>[4x]GSTLKEQIGMRALNVAETVASTSLVREAFRDSNPSVRLQPFAERIRQKTGAEYVVIGNRQGIAYAHPLTERIGKSMIGG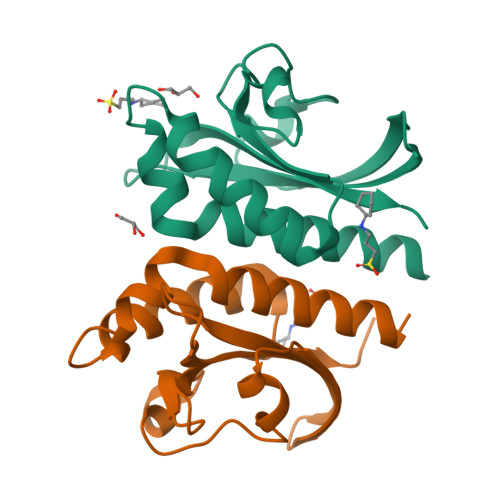DNKEVLKGKSIISEAVGSLGPAIRGKAPIFDENGSVIGIVSVGFLLEDIQRT> QRTVAHQITLLECVGKGRYGEVWRGSWQGENVAVKIFSSRDEKSWFRETELYNTVMLRHENILGFIASDMTSRHSSTQLWLITHYHEMGSLYDYLQLTTLDTVSCLRIVLSIASGLAHLHIEIFGTQGKPAIAHRDLKSKNILVKKNGQCCIADLGLAVMHSQ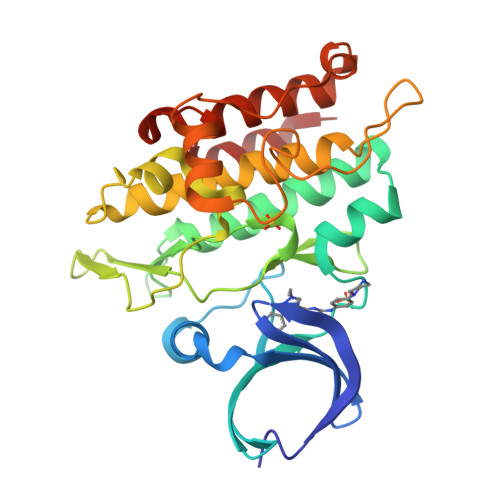STNQLDVGNNPRVGTKRYMAPEVLDETIQVDCFDSYKRVDIWAFGLVLWEVARRMVSNGIVEDYKPPFYDVVPNDPSFEDMRKVVCVDQQRPNIPNRWFSDPTLTSLAKLMKECWYQNPSARLTALRIKKTLTKID> 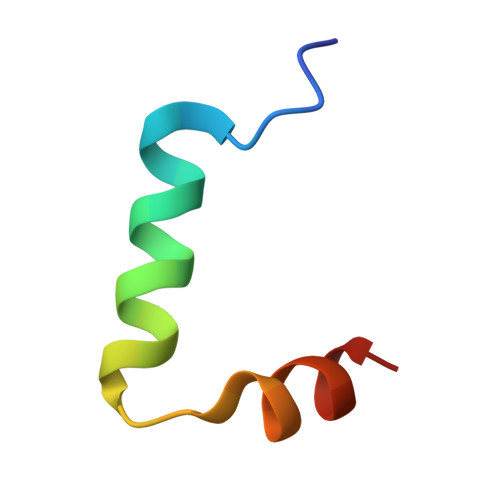MVSKLSQLQTELLAALLESGLSKEALIQALGE>GSTSAQEWQPVYPMSQLSFDRILKKDLVQGEHLGRGTRTHIYSGTLMDYKDDEGTSEEKKIKVILKVLDPSHRDISLAFFEAASMMRQVSHKHIVYLYGVC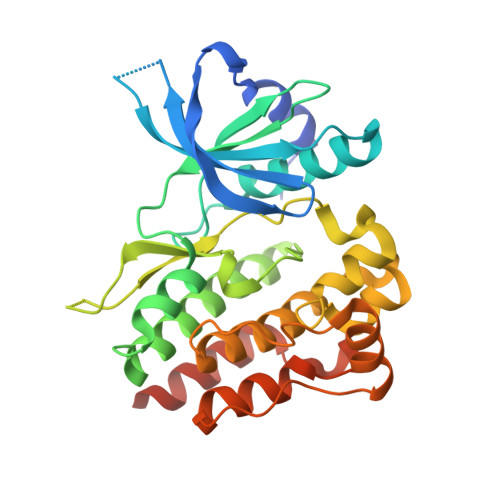FRDVENIMVEEFVEGGPLDLFMHRKSDVLTTPWKFKVAKQLASALSYLEDKDLVHGNVCTKNLLLAREGIDSECGPFIKLSDPGIPITVLSRQECIERIPWIAPECVEDSKNLSVAADKWSFGTTLWEICYNGEIPLKDKTLIEKERFYESRCRPVTPSCKELADLMTRCMNYDPNQRPFFRAIMRDINKLEEQNPDIVSEKK[2x]> QKPQRPRRPASPISTIQPKANFDAQQFAGTWLLVAVGSAGRFLQEQGHRAEATTLHVAPQGTAMAVSTFRKLDGICWQVRQLYGDTGVLGRFLLQARGARGAVHVVVAETDYQSFAVLYLERAGQLSVKLYARSLPVSDSVLSGFEQRVQEAHLTEDQIFYFPKYGFCEAADQFHV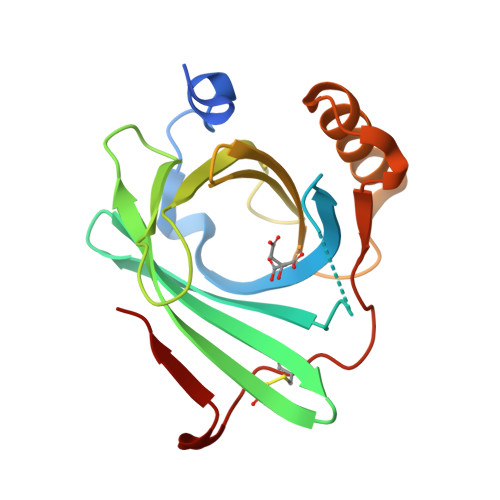LDEVRR> MGSSHHHHHHSQDPNSVRLAEELERQQLLEKRKKERNLHLQKINSIIDFIKERQSEQWSRQERCFQFGRLGASLHNQMEKDEQKRIEKTAKQRLAALKSNDEEAYLKLLDQTKDTRITQLLRQTNSFLDSLSEAVRAQQNEAKILHGEEVQPITDEEREKTDYYEVAHRIKEKIDKQPSILVGGTLKEYQLRGLEWMVSLYNNHLNGILADEMGLGKTIQSISLITYLYEVKKDIGPFLVIVPLSTITNWTLEFEKWAPSLNTIIYKGTPNQRHSLQHQIRVGNFDVLLTTYEYIIKDKSLLSKHDWAHMIIDEGHRMKNAQSKLSFTISHYYRTRNRLILTGTPLQNNLPELWALLNFVLPKIFNSAKTFEDWFNTPFANTGTQEKLELTEEETLLIIRRLHKVLRPFLLRRLKKEVEKDLPDKVEKVIKCKLSGLQQQLYQQMLKHNALFVGAGTEGATKGGIKGLNNKIMQLRKICNHPFVFDEVEGVVNPSRGNSDLLFRVAGKFELLDRVLPKFKASGHRVLMFFQMTQVMDIMEDFLRMKDLKYMRLDGST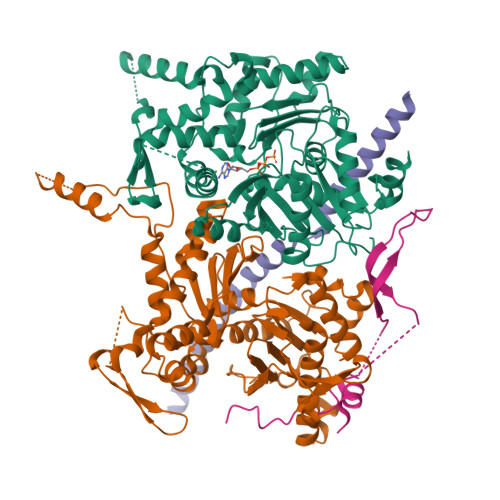KTEERTEMLNAFNAPDSDYFCFLLSTRAGGLGLNLQTADTVIIFDTDWNPHQDLQAQDRAHRIGQKNEVRILRLITTDSVEEVILERAMQKLDIDGKVIQAGKFDNKSTAEEQEAFLRRLIESETNRDDDDKAELDDDELNDTLARSADEKILFDKIDKERMNQERADAKAQGLRVPPPRLIQLDELPKVFREDIEEHFKKEDSEPLGRIRQKKRVYYDDGLTEEQFLEAVEDDNMSLEDAIKKRREARERRRLRQ;> MTLNRKCVVIHNGSHRTVAGFSNVELPQCIIPSSYIKRTDEGGEAEFIFGTYNMIDAAAEKRNGDEVYTLVDSQGLPYNWDALEMQWRYLYDTQLKVSPEELPLVITMPATNGKPDMAILERYYELAFDKLNVPVFQIVIEPLAIALSMGKSSAFVIDIGASGCNVTPIIDGIVVKNAVVRSKFGGDFLDFQVHERLAPLIKEENDMENMADEQKRSTDVWYEASTWIQQFKSTMLQVSEKDLFELERYYKEQADIYAKQQEQLKQMDQQLQYTALTGSPNNPLVQKKNFLFKPLNKTLTLDLKECYQFAEYLFKPQLISDKFSPEDGLGPLMAKSVKKAGASINSMKANTSTNPNGLGTSHINTNVGDNNSTASSSNISPEQVYSLLLTNVIITGSTSLIEGMEQRIIKELSIRFPQYKLTTFANQVMMDRKIQGWLGALTMANLPSWSLGKWYSKEDYETLKRDRKQSQATNATN;> MAPFRQDSILIIYPRSQTTLVQFGLNEETFTVPELEIPTQIYRTTRQDGSYTYHSTNKDNKAELIKPIQNGEIIDISAFTQFLRLIFVSILSDRANKNQDAFEAELSNIPLLLITHHSWSQSDLEIITQYVFESLEINNLIQLPASLAATYSMISLQNCCIIDVGTHHTDIIPIVDYAQLDHLVSSIPMGGQSINDSLKKLLPQWDDDQIESLKKSPIFEVLSDDAKKLSSFDFGNENEDEDEGTLNVAEIITSGRDTREVLEERERGQKVKNVKNSDLEFNTFWDEKGNEIKVGKQRFQGCNNLIKNISNRVGLTLDNIDDINKAKAVWENIIIVGGTTSISGFKEALLGQLLKDHLIIEPEEEKSKREEEAKSVLPAATKKKSKFMTNSTAFVPTIEYVQCPTVIKLAKYPDYFPEWKKSGYSEIIFLGAQIVSKQIFTHPKDTFYITREKYNMKGPAALWDVQF;> MDPQTLITKANKVSYYGNPTSKESWRYDWYQPSKVSSNVQQPQQQLGDMENNLEKYPFRYKTWLRNQEDEKNLQRESCEDILDLKEFDRRILKKSLMTSHTKGDTSKATGAPSANQGDEALSVDDIRGAVGNSEAIPGLSAGVNNDNTKESKDVKMN Transglutaminase 2 (TG2) is a GTP-binding, protein-crosslinking enzyme that has been investigated as a therapeutic target for Celiac disease, neurological disorders, and aggressive cancers. TG2 has been suggested to adopt two conformational states that regulate its functions: a GTP-bound, closed conformation, and a calcium-bound, crosslinking-active open conformation. The primary function of TG2 is to cross link proteins via the formation of amide bonds between glutamine residues and primary amine groups. Using SAXS and cryo-EM, we show that guanine nucleotides bind and stabilize a monomeric closed conformation while calcium binds to an open state that can form higher order oligomers.

X-ray crystallography structures of TG2 have revealed that GDP or GTP binds to a “closed” conformational state that occludes the protein-crosslinking (transamidation) active site and thus eliminates its crosslinking activity. Previous crystallographic studies of TG2 bound to GDP have shown that TG2 has a propensity to crystallize as a closed state dimer. To confirm that the structure of TG2 bound to guanine nucleotide is in fact a closed state monomer, we used cryo-EM to solve a 3.2 Å structure of TG2 bound to GDP. The cryo-EM structure of GDP-bound TG2 is in excellent agreement with the crystal structure with an overall RMSD of 0.8 Å; TG2 adopts the monomeric closed state and the cryo-EM map displays strong density for the nucleotide binding site and the bound GDP molecule. As described in crystallographic studies, GDP is stabilized through π-π stacking interactions of the guanine ring with Phe174 as well as several hydrogen bond interactions between the α and β phosphate of GDP and a trio of arginine residues, Arg476, Arg478, and Arg580. Importantly, due to the stabilizing interactions with Arg580 in wildtype TG2, GTP is able to bind to the closed state TG2 monomer by achieving a high-affinity interaction that can overcome the flexibility of the β-barrel domains. The SAXS experiments were carried out at 25 µM TG2 to achieve a sufficient scattering signal, while the cryo-EM analysis was carried out using 3 µM TG2 as was necessary to obtain an appropriate particle density, which made it possible to capture the monomeric form of the TG2 open state.

> MAEELVLERCDLELETNGRDHHTADLCREKLVVRRGQPFWLTLHFEGRNYEASVDSLTFSVVTGPAPSQEAGTKARFPLRDAVEEGDWTATVVDQQDCTLSLQLTTPANAPIGLYRLSLEASTGYQGSSFVLGHFILLFNAWCPADAVYLDSEEERQEYVLTQQGFIYQGSAKFIKNIPWNFGQFEDGILDICLILLDVNPKFLKNAGRDCSRRSSPVYVGRVVSGMVNCNDDQGVLLGRWDNNYGDGVSPMSWIGSVDILRRWKNHGCQRVKYGQCWVFAAVACTVLRCLGIPTRVVTNYNSAHDQNSNLLIEYFRNEFGEIQGDKSEMIWNFHCWVESWMTRPDLQPGYEGWQALDPTPQEKSEGTYCCGPVPVRAIKEGDLSTKYDAPFVFAEVNADVVDWIQQDDGSVHKSINRSLIVGLKISTKSVGRDEREDITHTYKYPEGSSEEREAFTRANHLNKLAEKEETGMAMRIRVGQSMNMGSDFDVFAHITNNTAEEYVCRLLLCARTVSYNGILGPECGTKYLLNLNLEPFSEKSVPLCILYEKYRDCLTESNLIKVRALLVEPVINSYLLAERDLYLENPEIKIRILGEPKQKRKLVAEVSLQNPLPVALEGCTFTVEGAGLTEEQKTVEIPDPVEAGEEVKVRMDLLPLHMGLHKLVVNFESDKLKAVKGFRNVIIGPA>[2x]KVTMNDFDYLKLLGKGTFGKVILVREKATGRYYAMKILRKEVIIAKDEVAHTVTESRVLQNTRHPFLTALKYAFQTHDRLCFVMEYANGGELFFHLSRERVFTEERARFYGAEIVSALEYLHSRDVVYRDIKLENLMLDKDGHIKITDFGLCKEGISDGATMKTFCGTPEYLAPEVLEDNDYGRAVDWWGLGVVMYEMMCGRLPFYNQDHERLFELILMEEIRFPRTLSPE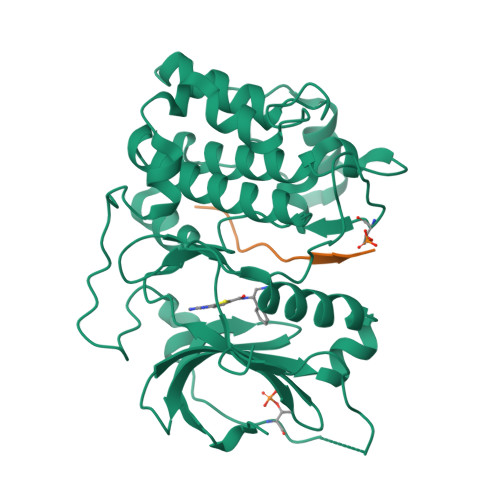AKSLLAGLLKKDPKQRLGGGPSDAKEVMEHRFFLSINWQDVVQKKLLPPFKPQVTSEVDTRYFDDEFTAQSITITPPDRYDSLGLLELDQRTHFPQFDYSASIR;>[2x]GRPRTTSFAE>[4x]MRILVTNDDGIYSPGLWALAEAASQFGEVFVAAPDTEQSAAGHAITIAHPVRAYPHPSPLHAPHFPAYRVRG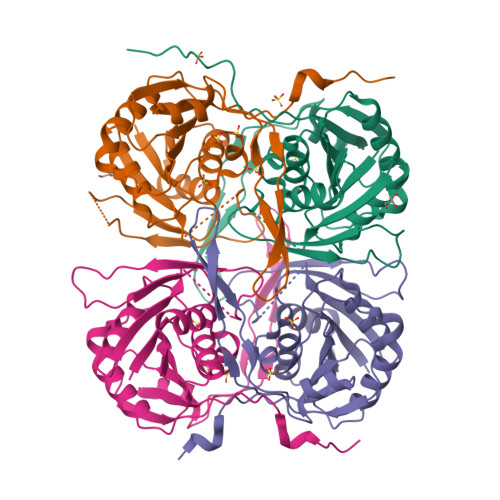TPADCVALGLHLFGPVDLVLSGVNLGSNLGHEIWHSGTVAAAKQGYLFGLSAAAFSVPLNGEVPDFAGLRPWLLRTLETLLRLERPFLVNVNLPLRPKGFLWTRQSVRAYEGVVIPGEDPMGRPFYWFAPRPLKEAEEGTDRWAVAQGFVSATPLRLDLTDETRLQPTLAHD> MAAVAAVAARRRRSWASLVLAFLGVCLGITLAVDRSNFKTCEESSFCKRQRSIRPGLSPYRALLDSLQLGPDSLTVHLIHEVTKVLLVLELQGLQKNMTRFRIDELEPRRPRYRVPDVLVADPPIARLSVSGRDENSVELTMAEGPYKIILTARPFRLDLLEDRSLLLSVNARGLLEFEHQRAPRVSQGSKDPAEGDGAQPEETPRDGDKPEETQGKAEKDEPGAWEETFKTHSDSKPYGPMSVGLDFSLPGMEHVYGIPEHADNLRLKVTEGGEPYRLYNLDVFQYELYNPMALYGSVPVLLAHNPHRDLGIFWLNAAETWVDISSNTAGKTLFGKMMDYLQGSGETPQTDVRWMSETGIIDVFLLLGPSISDVFRQYASLTGTQALPPLFSLGYHQSRWNYRDEADVLEVDQGFDDHNLPCDVIWLDIEHADGKRYFTWDPSRFPQPRTMLERLASKRRKLVAIVDPHIKVDSGYRVHEELRNLGLYVKTRDGSDYEGWCWPGSAGYPDFTNPTMRAWWANMFSYDNYEGSAPNLFVWNDMNEPSVFNGPEVTMLKDAQHYGGWEHRDVHNIYGLYVHMATADGLRQRSGGMERPFVLARAFFAGS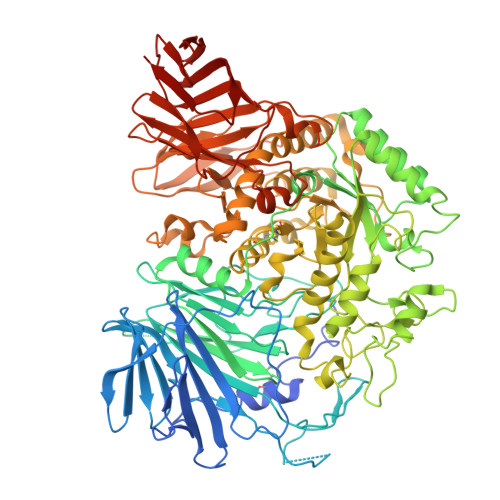QRFGAVWTGDNTAEWDHLKISIPMCLSLGLVGLSFCGADVGGFFKNPEPELLVRWYQMGAYQPFFRAHAHLDTGRREPWLLPSQHNDIIRDALGQRYSLLPFWYTLLYQAHREGIPVMRPLWVQYPQDVTTFNIDDQYLLGDALLVHPVSDSGAHGVQVYLPGQGEVWYDIQSYQKHHGPQTLYLPVTLSSIPVFQRGGTIVPRWMRVRRSSECMKDDPITLFVALSPQGTAQGELFLDDGHTFNYQTRQEFLLRRFSFSGNTLVSSSADPEGHFETPIWIERVVIIGAGKPAAVVLQTKGSPESRLSFQHDPETSVLVLRKPGINVASDWSIHLR>MRGSHHHHHHGSACELSECPVRKSNVGGGGTRNHDWWPAQLRLNILRQHTPVSNPLDKDFDYAAAFKSLDYEGLKKDLTKLMTDSQDWWPADFGHYGGLFIRMAXHSAGTYRVTDGRGGGGEGQQRFAPLNSWPDNVSLDKARRLLWPIKQKYGNKISWSDLLLLTGNVALESMGFKTFGFAGGRPDTWEADESVYWGAETTWLGNEDRYSEGQEGHEGHGVVQGDESKKQHTDIHNRDLQSPLASSHMGLIYVNPEGPDGIPDPVASAKDIRVTFGRMAMNDEETVALIAGGHSFGKTHGAGPTHHVGKEPEAAPIEHQGLGWANSFGQGKGPDTITSGLEVTWTPTPTKWGMGYLEYLYKFDWEPTKSPAGANQWVAKNAEPTIPDAYDPNKKKLPTMLTTDIALRMDPAYDKICRDYLANPDKFADAFARAWFKLLHRDMGPRTRWIGPEVPSEILPWEDYIPPVDYQIIDDNDIAALKKEILATGVAPKKLIFVAWSSASSFRGSDKRGGANGARIRLAPQNEWKVNDPSTLREVLAALESVQQKFNDSSSGKKVSLADLIVLGGVAALEQASGLVVPFTPGRNDATQEHTDVHSFTHLEPHADGFRSYGKGTKR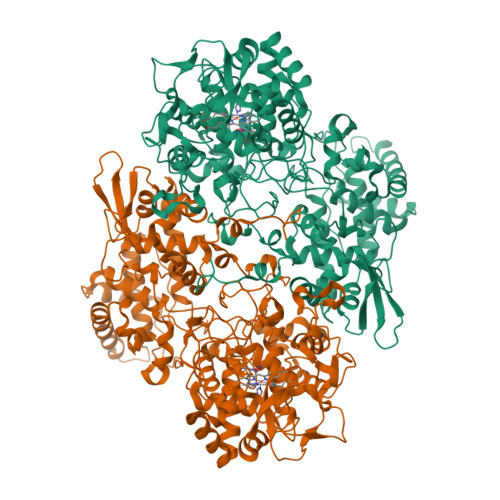VRTEQFLIDRASLLTLSAPELTALIGGLRVLEANYDGSSYGVLTKTPGKLTNDYFVNLLDTNTAWKAADNEGEVFIGYDRKTHDKKWTATRADLIFGAHAELRALAEVYAAVDGEEKFKRDFVAAWHKVMNLDRFDLKQEGRGQNAPKL[2x]>MASWSHPQFEKGADDDDKVPDPTSVDAVKHNRIKGIPKLDDANDAGGRNSTECTLILTEGDSAKTLAVSGLGVVGRDKYGVFPLRGKILNVREASHKQIMENAEINNIIKIVGLQYKKNYEDEDSLKTLRYGKIMIMTDQDQDGSHIKGLLINFIHHNWPSLLRHRFLEEFITPIVKVSKNKQEMAFYSLPEFEEWKSSTPNHKKWKVKYYKGLGTSTSKEAKEYFADMKRHRIQFKYSGPEDDAAISLAFSKKQIDDRKEWLTNFMEDRRQRKLLGLPEDYLYGQTTTYLTYNDFINKELILFSNSDNERSIPSMVDGLKPGQRKVLFTCFKRNDKREVKVAQLAGSVAEMSSYHHGEMSLMMTIINLAQNFVGSNNLNLLQPIGQFGTRLHGGKDSASPRYIFTMLSSLARLLFPPKDDHTLKFLYDDNQRVEPEWYIPIIPMVLINGAEGIGTGWSCKIPNFDVREIVNNIRRLMDGEEPLPMLPSYKNFKGTIEELAPNQYVISGEVAILNSTTIEISELPVRTWTQTYKEQVLEPMLNGTEKTPPLITDYREYHTDTTVKFVVKMTEEKLAEAERVGLHKVFKLQTSLTCNSMVLFDHVGCLKKYDTVLDILRDFF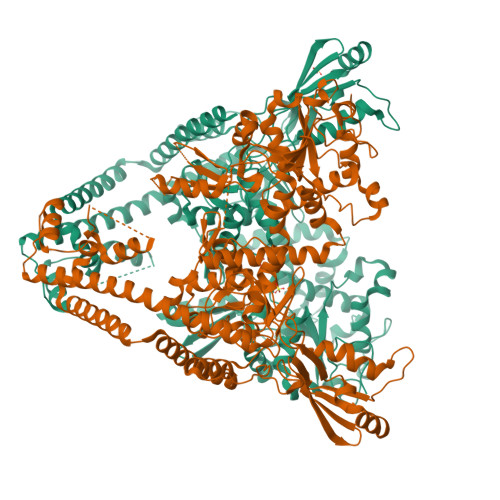ELRLKYYGLRKEWLLGMLGAESAKLNNQARFILEKIDGKIIIENKPKKELIKVLIQRGYDSDPVKAWKEAQQKVPDEEENEESDNEKETEKSDSVTDSGPTFNYLLDMPLWYLTKEKKDELCRLRNEKEQELDTLKRKSPSDLWKEDLATFIEELEAVEAKEKQDGAPGFSSISAHHHHHHHHHH[4x]>[2x]MEIVEYPDPILRAKNKR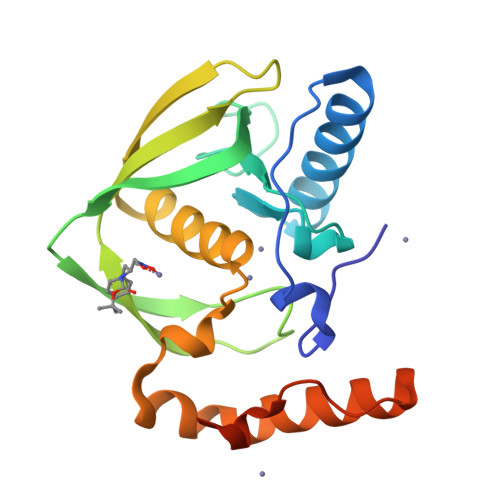IDIFDENLKNLVDAMFDVMYKTDGIGLSAPQVGLNVQLMVFNPAGEPGEGKEIVLVNPKIKKYSDKLVPFDEGCLSFPGIYAEVVRPQSVKIDARDITGERFSISLSRLPARIFQHEYDHLEGVLFFDRMTDQVLDSIREELEALEKKYEEKTGLPSPERVEARQKRKAGVGFGKR> ATGGYVQQATGQASFTMYSGCGSPACGKAASGFTAAINQLA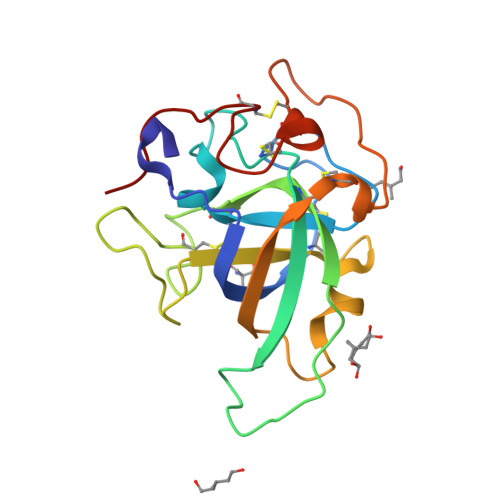FGSAPGLGAGDACGRCFALTGNHDPYSPNYTGPFGQTIVVKVTDLCPVQGDQEFCGQTTSNPTNQHGMPFHFDICEDTGGSAKFFPSGHGALTGTFTEVSCSQWSGSDGGQLWNGACLSGETAPNWPSTACGNKGTAPS>GPLGSKQVFKNRKYPITDFEKYLQDITKVRGPMSIDTFIKEVLTNPKYGYYMNKDVFGKGGDFITAPEVSQLFGEMIGIWCVATWEAMGKPKKLQIVEMGPGRGTLMKDILRSTKVFKEFYDSISVHLVEASPANKKTQKQNLLYFKDKAINFDHKTIGETPNGIKVTWVGKLEEVPTDIPTLFLAQEFFDALPIHVFRFSREKNDWCEVLVDEDITEHGEYYLRFVQSKGPTLMTTAVKHLLPEFGLDGYQVELGLAGLAISQQIANRIDKSG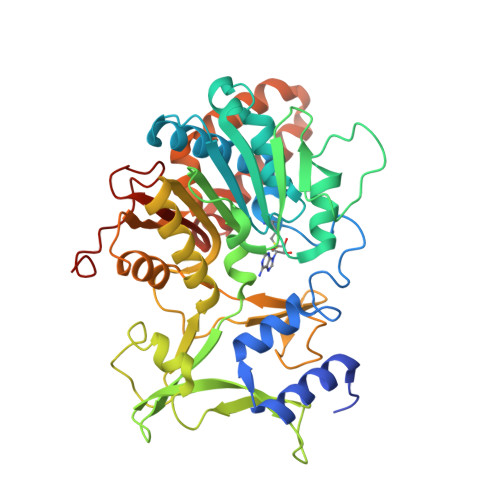GAALIIDYGYDKIVKSSLQAIRDHEFVDILDKPGTADLSVWVDFQTIRKTVKLLKNKSTAIGPVDQGIFLKEMGIEHRLAQIGRKLDSNEKFEELVMGYKKLVDPKEMGTNYKVITICDKNITPIGFSTSKTYDDEDLMI[3x]>[2x]MVSPQTRKEEELLEKQNSVFYLLTLGRK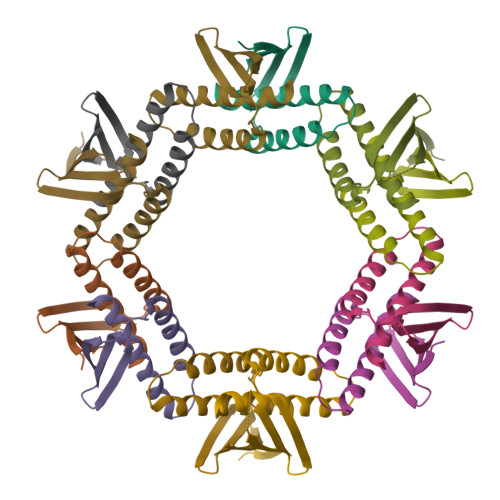PYGSYLHIKIELDEDEKLEKEIYADNIKLENELRQLKRLYEVYQSVEIDDAQKAIQKEALLTIAKILSVFDFHHHHHH>GKQLTILGSTGSIGCSTLDVVRHNPEHFRVVALVAGKNVTRMVEQCLEFSPRYAVMDDEASAKLLKTMLQQQGSRTEVLSGQQAACDMAALEDVDQVMAAIVGAAGLLPTLAAIRAGKTILLANKESLVTCGRLFMDAVKQSKAQLLPVDSEHNAIFQSLPQPIQHNLGYADLEQNGVVSILLTGSGGPFRETPLRDLATMTPDQACRHPNWSMGRKISVDSATMMNKGLEYIEARWLFNASASQMEVLIHPQSVIHSMVRYQDGSVLAQLGEPDMRTPIAHTMAWPNRVNSGVKPLDFCKLSALTFAAPDYDRYPCLKLAMEAFEQGQAATTALNAANEITVAAFLAQQIRFTDIA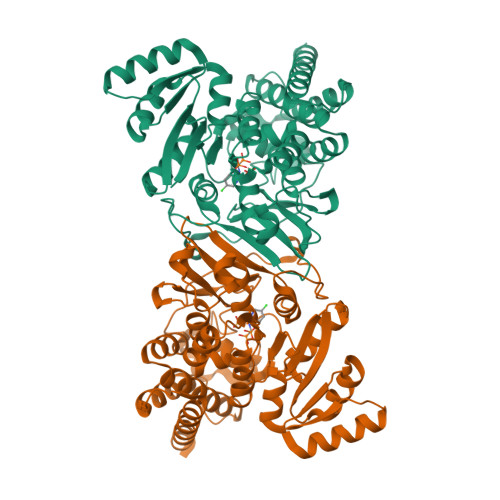ALNLSVLEKMDMREPQCVDDVLSVDANAREVARKEVMRLAS[2x]>TVPDRDNDGIPDSLEVEGYTVDVKNKRTFLSPWISNIHEKKGLTKYKSSPEKWSTASDPYSDFEKVTGRIDKNVSPEARHPLVAAYPIVHVDMENIILSKNEDQSTQNTDSQTRTISKNTSTSRTHTSEVHGNAEVHASFFDIGGSVSAGFSNSNSSTVAIDHSLSLAGERTWAETMGLNTADTARLNANIRYVNTGTAPIYNVLPTTSLVLGKNQTLATIKAKENQLSQILAPNNYYPSKNLAPIALNAQDDFSSTPITMNYNQFLELEKTKQLRLDTDQVYGNIATYNFENGRVRVDTGSNWSEVLPQIQETTARIIFNGKDLNLVERRIAAVNPSDPLETTKPDMTLKEALKIAFGFNEPNGNLQYQGKDITEFDFNFDQQTSQNIKNQLAELNATNIYTVLDKIKLNAKMNILIRDKRFHYDRNNIAVGADESVVKEAHREVINSSTEGLLLNIDKDIRKILSGYIVEIEDTEGLKEVINDRYDMLNISSLRQDGKTFIDFKKYNDKLPLYISNPNYKVNVYAVTKENTIINPSENGDTSTNGIKKILIFSKKGYEIG[7x];> AGGHGDVGMHVKEKEKNKDENKRKDEERNKTQEEHLKEIMKHIVKIEVKGEEAVKKEAAEKLLEKVPSDVLEMYKAIGGKIYIVDGDITKHISLEALSEDKKKIKDIYGKDALLHEHYVYAKEGYCPVLVIQSSEDYVENTEKALNVYYE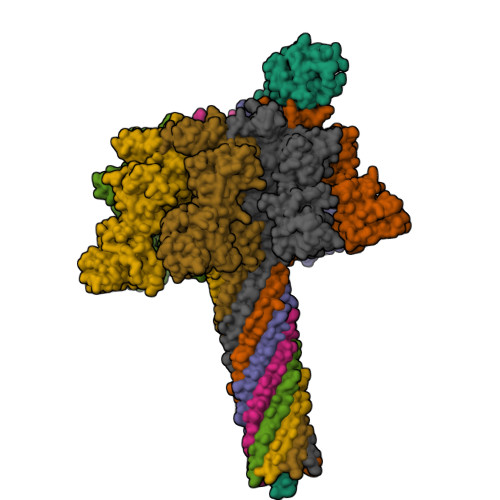IGKILSRDILSKINQPYQKFLDVLNTIKNASDSDGQDLLFTNQLKEHPTDFSVEFLEQNSNEVQEVFAKAFAYYIEPQHRDVLQLYAPEAFNYMDKFNEQEINLSLEELKDQR>MKIDESLNVHSSLLQLIGNTPLLELHKITKGLKGRYFAKLEAFNVGHSAKDRVAKYIVEDAERKGLLKPGSTIVETSSGNTGYSLAMISALRGYRCIIAISDKSSHDKVEMLQALGAEVHLCPANVAPDDPRSYYEVAKRIHNETPNSIYVNQYFNPLNPESHYQTGREIWEQTQGEITHVVVCSGTGGTISGIAHYLKEQNPRVQVLGVDAYGSAIK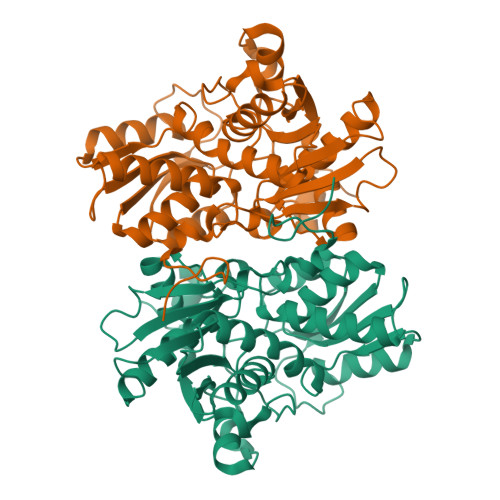KYHETREFDPAEVYPYKIEGIGKNLIPTATDFDVIDEFIKVTDKDAALMARKLARTEGLFMGYTSGAAIQAVKQYAEAGKFDENSIVVVLFADHGSRYMNKIYSDDWMKKQGFID[2x]>[4x]MVTAFILMVTAAGKEREVMEKLLAMPEVKEAYVVYGEYD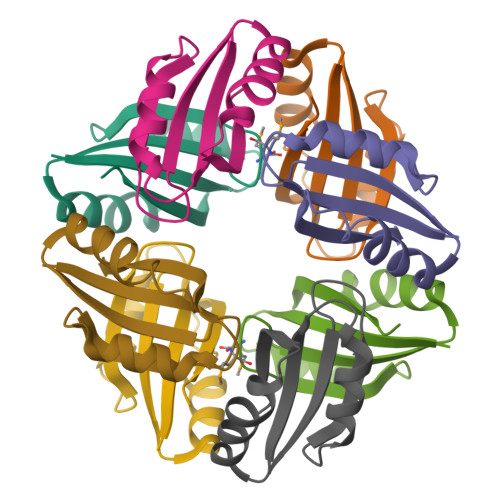LIVKVETDTLKDLDQFITEKIRKMPEIQMTSTMIAI>APPPVPKTPAGPLTLSGQGSFFVGGRDVTSETLSLSPKYDAHGTVTVDQMYVRYQIPQRAKRYPITLIHGCCLTGMTWETTPDGRMGWDEYFLRKGYSTYVIDQSGRGRSATDISAINAVKLGKAPASSLPDLFAAGHEAAWAIFRFGPRYPDAFKDTQFPVQAQAELWQQMVPDWLGSMPTPNPTVANLSKLAIKLDGTVLLSHSQSGIYPFQTAAMNPKGITAIVSVEPGECPKPED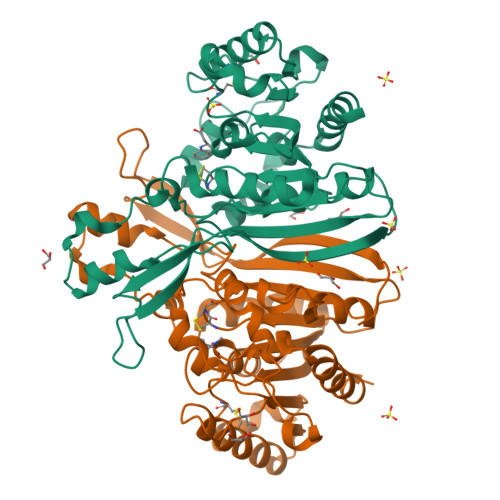VKPLTSIPVLVVFGDHIEEFPRWAPRLKACHAFIDALNAAGGKGQLMSLPALGVHGNSHMMMQDRNNLQVADLILDWIGRNTAKPAHGR[2x]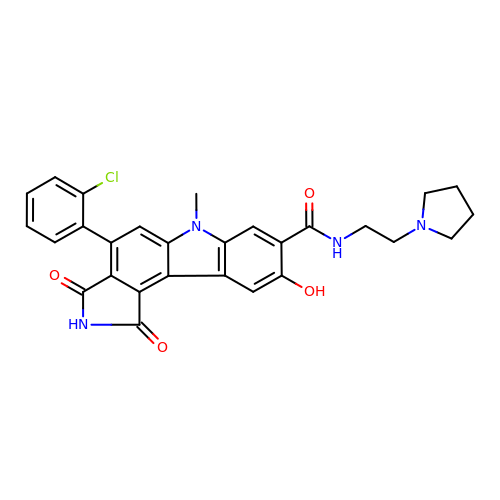4-(2-chlorophenyl)-9-hydroxy-6-methyl-1,3-dioxo-N-(2-pyrrolidin-1-ylethyl)pyrrolo[3,4-g]carbazole-8-carboxamide | C28 H25 Cl N4 O4 | LFRLUVCEFWYSFT-UHFFFAOYSA-N> MACRQEPQPQGPPPAAGAVASYDYLVIGGGSGGLASARRAAELGARAAVVESHKLGGTCVNVGCVPKKVMWNTAVHSEFMHDHADYGFPSCEGKFNWRVIKEKRDAYVSRLNAIYQNNLTKSHIEIIRGHAAFTSDPKPTIEVSGKKYTAPHILIATGGMPSTPHESQIPGASLGITSDGFFQLEELPGRSVIVGAGYIAVEMAGILSALGSKTSLMIRHDKVLRSFDSMISTNCTEELENAGVEVLKFSQVKEVKKTLSGLEVSMVTAVPGRLPVMTMIPDVDCLLWAIGRVPNTKDLSLNKLGIQTDDKGHIIVDEFQNTNVKGIYAVGDVCGK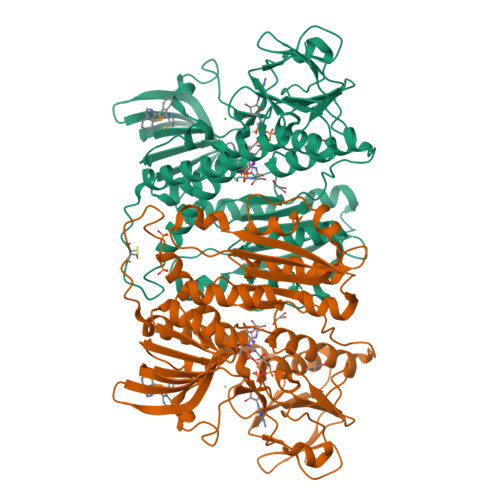ALLTPVAIAAGRKLAHRLFEYKEDSKLDYNNIPTVVFSHPPIGTVGLTEDEAIHKYGIENVKTYSTSFTPMYHAVTKRKTKCVMKMVCANKEEKVVGIHMQGLGCDEMLQGFAVAVKMGATKADFDNTVAIHPTSSEELVTLR> KNYTDYFFDEPAFDLHDGGYVPLEVSDAPEKPLNVPPLLKPDKETATDVYYTVTAEAGETQLLPGAKTKTWGYNTSLLGQTIVYRRGQHTHVTLKNTLPELTTFHWHGANVSGPYVDGGCHAPVYPGESKHIDFTLEQPATTLWLHAHPCPSTAEQVWHGLAAMVIVKDDHEASLPLPRNYGVDDIPVILQDRRFHENNQWDYRA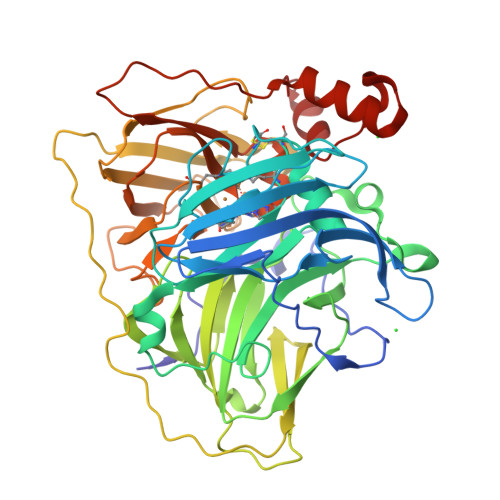DYDPDGVAGPTAMINGTINPYFDVTTQKVRLRFLNGANRREWRLHFADDLPFTQIGGDGSLLPEPVKFTHLMLTCAERAEVIVDFGQYHEGDEVTLYTDDVPLLKFRIHAFKPDQTTLPDKLFDVKAPVVDPALPVRHVVMQGMDEGVAIDGKKFAMQRIDATQPIGKAQYWDVTNSNDAPGMVHPFHVHGTQFLVLSRNGHAPYPNEHGFKDTIGVNPGETVRLLVRFDLPGVYMYHCHIIEHEDGGMMAQIETFDPAKPKQEYKLMDMDTLMMALAKERGVKPSEIWMGGMQSYEKMGMKM> MILVNKETRVLVQGITGREGQFHTKQMLSYGTKIVAGVTPGKGGMEVLGVPVYDTVKEAVAHHEVDASIIFVPAPAAADAALEAAHAGIPLIVLITEGIPTLDMVRAVEEIKALG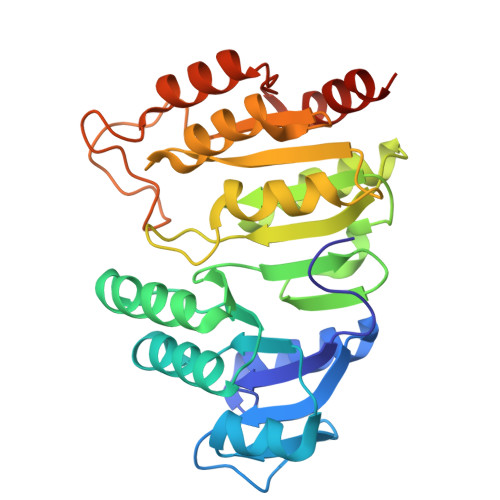SRLIGGNCPGIISAEETKIGIMPGHVFKRGRVGIISRSGTLTYEAAAALSQAGLGTTTTVGIGGDPVIGTTFKDLLPLFNEDPETEAVVLIGEIGGSDEEEAAAWVKDHMKKPVVGFIGGRSAPKGKRMGHAGAIIMGNVGTPESKLRAFAEAGIPVADTIDEIVELVKKALGWNSRPGIL>MTRFEIRDDFYLDGKSFKILSGAIHYFRVPPEDWYHSLYNLKALGFNTVETYVAWNLHEPCEGEFHFEGDLDLEKFLQIAQDLGLYAIVRPSPFICAEWEFGGLPAWLLTKNMRIRSSDPAYIEAVGRYYDQLLPRLVPRLLDNGGNILMMQVENEYGSYGEDKAYLRAIRQLMEECGVTCPLFTSDGPWRATLKAGTLIEEDLFVTGNFGSKAPYNFSQMQEFFDEHGKKWPLMCMEFWDGWFNRWKEPIITRDPKELADAVREVLEQGSINLYMFHGGTNFGFMNGCSARGTLDLPQVTSYDYDALLDEEGNPTAKYLAVKKMMATHFSEYPQLEPLYKESMELDAIPLVEKVSLFETLDSLSSPVESLYPQKMEELGQSYGYLLYRTETNWDAEEERLRIIDGRDRAQLYVDGQWVKTQYQTEIGEDIFYQGKKKGLSRLDILIENMGRVNYGHKFLADTQRKGIRTGVCKDLHFLLNWKHYPLPLDNPEKIDFSKGWTQGQPAFYAYDFTVEEPKDTYLDLSEFGKGVAFVNGQNLGRFWNVGPTLSLYIPHSYLKEGANRIIIF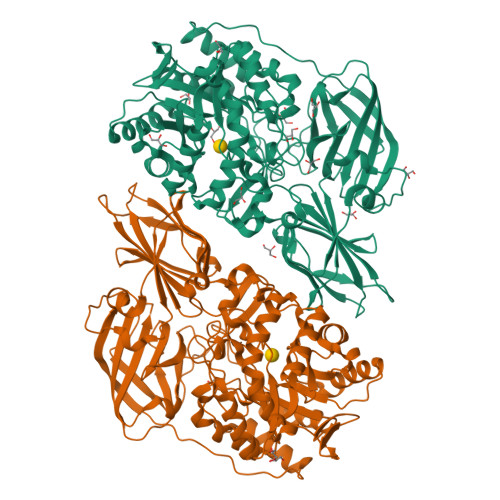ETEGQYKEEIHLTRKPTLKHIKGENL[2x]> MEKQVIQSVGFRNIKNGNGEITGFQFKVKLPYYRGVF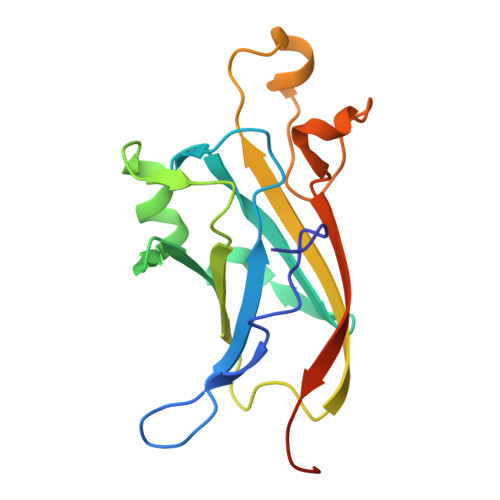LSQIRPGTLFVDGQKIEKDQITWTINGEEYTNQEMRGDFKTHWATTKPAVLKVKMPGGLAQGYHDLKYGFCFTSSYMPPIIQDGLDPDKESMVYMPEFGHHVNERRLLIVKLAAALEHHHHHH> AMKPRIYVKVKPERLGAVIGPRGEVKAEIMRRTGTVITVDTENSMVIVEPEAEGIPPVNLMKAAEVVKAISLGFPPEKAFRLLEE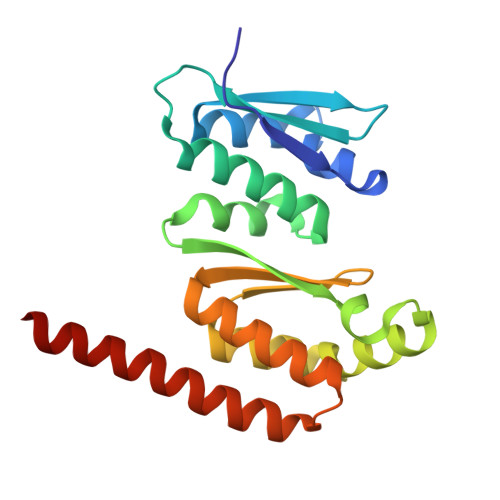DQILVVVDLKQVVGDSQNHLKRIKGRIIGEGGRARRTIEEMTDTYINVGEYEVAIIGDYERAMAAKQAIEMLAEGRMHSTVYRHLERIMREIKRRERLKMWAREEL>SSGVFELKLQEFVNKKGLLGNRNCCRGGAGPPPCACRTFFRVCLKHYQASVSPEPPCTYGSAVTPVLGVDSFSLPDGGGADSAFSNPIRFPFGFTWPGTFSLIIEALHTDSPDDLATENPERLISRLATQRHLTVGEEWSQDLHSSGRTDLKYSYRFVCDEHYYGEGCSVFCRPRDDAFGHFTCGERGEKVCNPGWKGPYCTEPICLPGCDEQHGFCDKPGECKCRVGWQGRYCDECIRYPGCLHGTCQQPW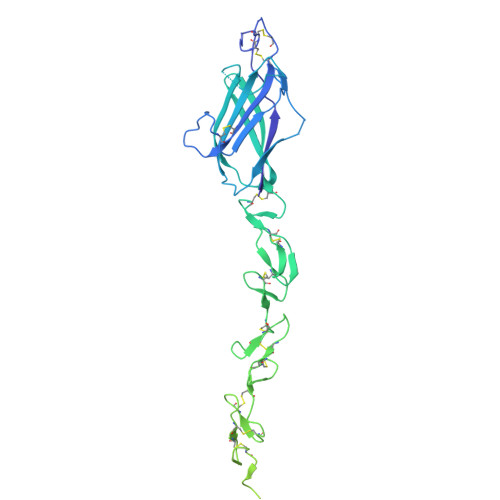QCNCQEGWGGLFCNQDLNYCTHHKPCKNGATCTNTGQGSYTCSCRPGYTGATCELGIDECDPSPCKNGGSCTDLENSYSCTCPPGFYGKICELSAMTCADGPCFNGGRCSDSPDGGYSCRCPVGYSGFNCEKKIDYCSSSPCSNGAKCVDLGDAYLCRCQAGFSGRHCDDNVDDCASSPCANGGTCRDGVNDFSCTCPPGYTGRNCSAPVSRCEHAPCHNGATCHQRGHGYVCECARSYGGPNCQFLLPELPPGPAVVDLTEKLEGQGGPFPWENLYFQ[2x]>MNKTDLINAVAEQADLTKKEAGSAVDAVFESIQNSLAKGEKVQLIGFGNFEVRERAARKGRNPQTGKEIDIPAS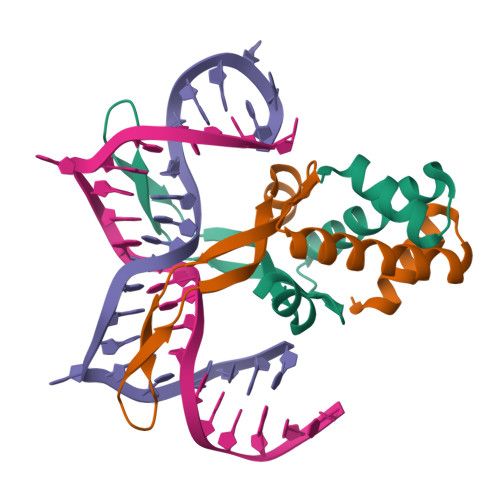KVPAFKAGKALKDAVKLEHHHHHH[2x]>[2x]MEEAVLTGVATDKSEAKVTVLGISDKPGE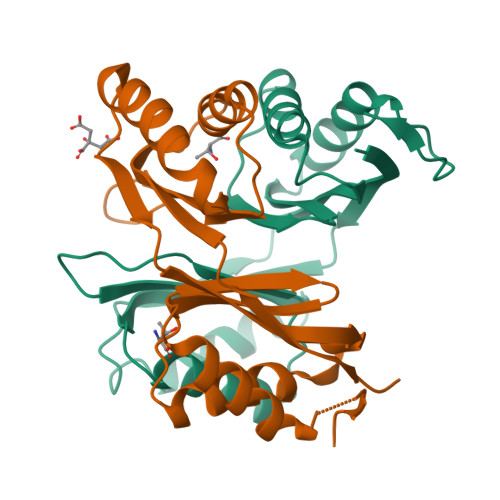AAKVFRALADAEINIDMVLQNVSSVEDGTTDITFTCPRSDGRRAMEILKKLQVQGNWTNVLYDDQVGKVSLVGAGMKSHPGVTAEFMEALRDVNVNIELISTSEIRISVLIREDDLDAAARALHEQFQLGGEDEAVVYAGTGRHHHHHH> MSVIKSDMKIKLRMEGTVNGHKFVIEGEGEGKPYEGTQTMNLKVKEGAPLPFAYDILTTAFHYGNRVFAKYPKDIPDYFKQSFPEGYSWERSMTFEDGGICTARNDITLEGDCFFNEIRFDGVNFPPNGPVMQKKTLKWEPSTEKMYVRDGVLMGDVNMALLLEGGGHYRCDFKTTYKAKKGVQLPDYHFVDHCIEILS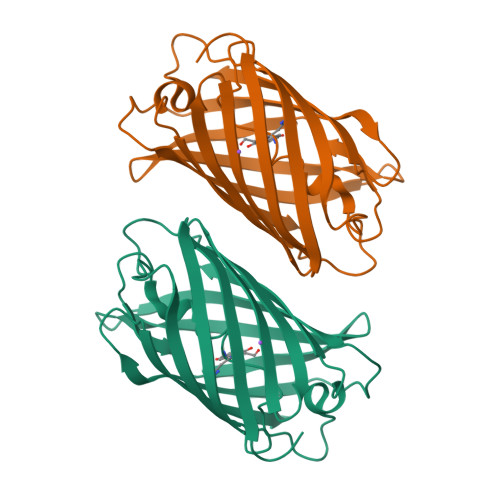HDKDYNNVKLYEHAVAHSGLPRQAKHHHHHH> XRMKQIEDKIEEIESKQKKIENEIAR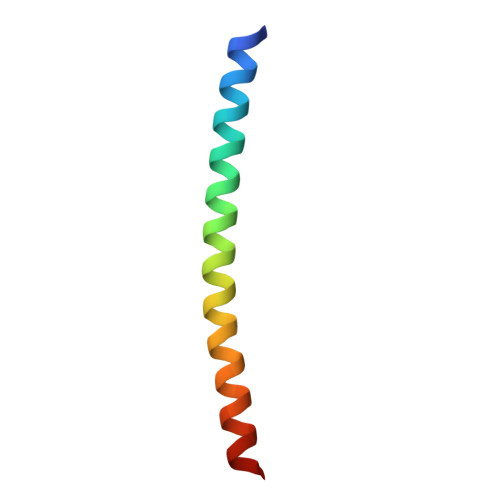IKKLLQLTVWGIKQLQARILX N~5~-[(3-(ethylsulfanyl)propanimidoyl]-L-ornithine | C10 H21 N3 O2 S | 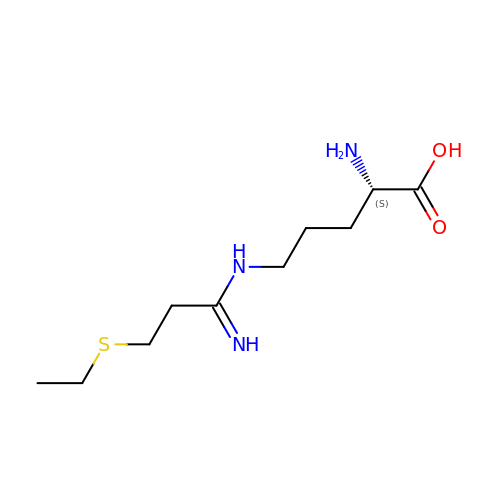HAZXKSBWYNTCGM-QMMMGPOBSA-N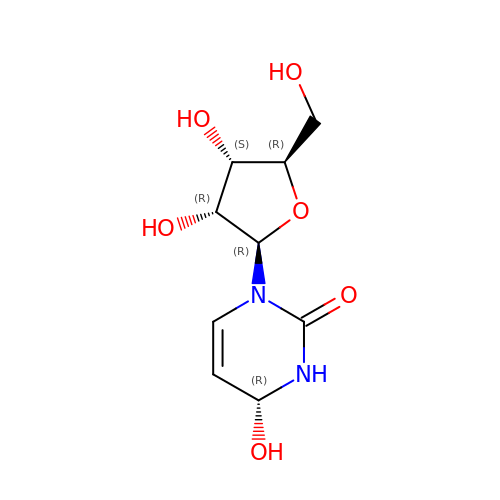4-HYDROXY-3,4-DIHYDRO-ZEBULARINE | C9 H14 N2 O6 | LUOTYVSEHPPZEM-FMDGEEDCSA-N>[2x]GPLGSGSGHLAIGSAATLGSGGMARGREPGGVGHVVAQVQSVDGNAQCCDCREPAPEWASINLGVTLCIQCSGIHRSLGVHFSKVRSLTLDSWEPELVKLMCELGNVIINQIYEARVEAMAVKKPGPSCSRQEK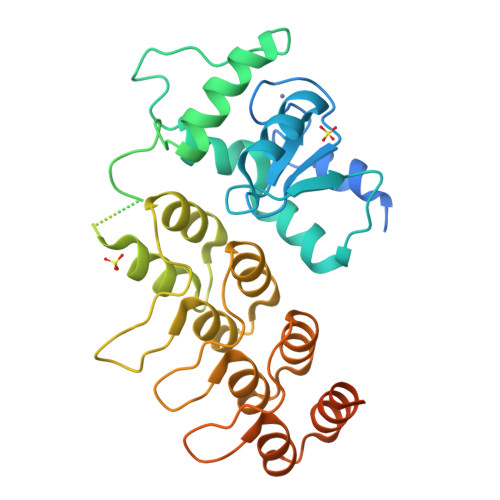EAWIHAKYVEKKFLTKLPEIRGRRGGRGRPRGQPPVPPKPSIRPRPGSLRSKPEPPSEDLGSLHPGALLFRASGHPPSLPTMADALAHGADVNWVNGGQDNATPLIQATAANSLLACEFLLQNGANVNQADSAGRGPLHHATILGHTGLACLFLKRGADLGARDSEGRDPLTIAMETANADIVTLLRLAKMREAEAAQGQAGDETYLDIFRDFSLMASDDPEKLSRRSHDLHTL>MESRDHNNPQEGPTSSSGRRAAVEDNHLLIKAVQNEDVDLVQQLLEGGANVNFQEEEGGWTPLHNAVQMSREDIVELLLRHGADPVLRKKNGATPFILAAIAGSVKLLKLFLSKGADVNECDFYGFTAFMEAAVYGKVKALKFLYKRGANVNLRRKTKEDQERLRKGGATALMDAAEKGHVEVLKILLDEMGADVNACDNMGRNALIHALLSSDDSDVEAITHLLLDHGADVNVRGERGKTPLILAVEKKHLGLVQRLLEQEHIEINDTDSDGKTALLLAVELKLKKIAELLCKRGASTDCGDLVMTARRNYDHSLVKVLLSHGAKEDFH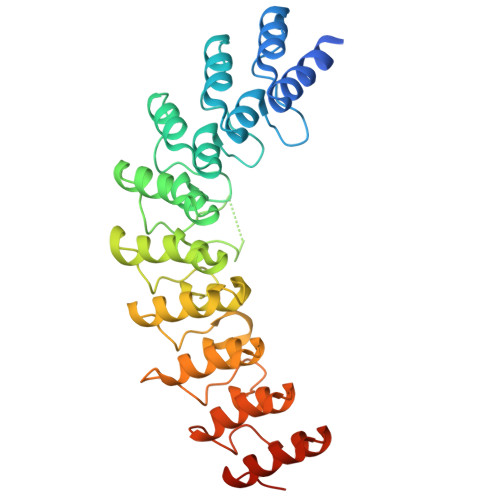PPAEDWK[2x]>[2x]HHHHHHMKRIHIVAGIIFNSDQSEIFITKRPDHLHKGGFWEFPGGKVEAG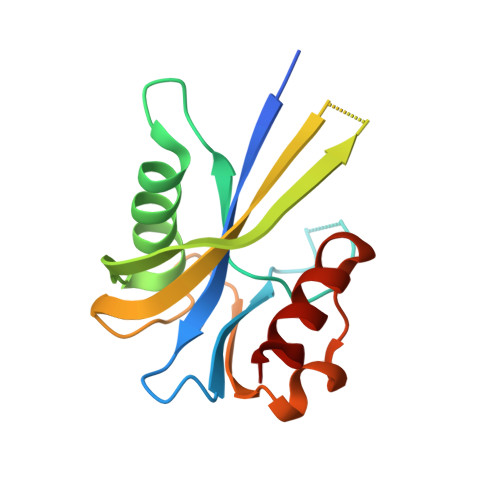ESREQAMVRELEEEIGITVTEQQAFQHFDFDYTDKSLSFDFMLVTAFDGQPHGREGQQGGWVKIADLANYRFPEANDPVVKQVIAQFG Here we analyze by comparative genomics Pb mosquitocidal and non-mosquitocidal strains and show that the active component in Pbm responsible for Anopheles toxicity is a complex that contains a clostridial neurotoxin (CNT) that has high selectivity to anopheline mosquitoes, acquired through a megaplasmid. We found a second toxin locus (ptox) flanked by insertion sequences and transposon elements. This locus encodes a protein, which we named paraclostridial mosquitocidal protein 1 (PMP1), with high similarity to CNTs, a group that includes the tetanus neurotoxin (TeNT) and botulinum neurotoxins (BoNTs). PMP1’s closest relative is BoNT/X from C. botulinum strain 111 (36% identity), followed by BoNT/En, the Enterococcus BoNT-like protein7,9 (34% identity). PMP1 presents the conserved SxWY motif in the binding domain (HC), which in BoNTs is involved in ganglioside receptor binding (Supplemenatry Fig. 1C), as well as the conserved disulfide bond that links the toxin heavy and light chains, and is essential for toxicity. PMP1 is thus the first CNT that targets invertebrates.

To analyze if the SxWY motif is involved in toxicity and to determine the presence of other cell recognition regions, recombinant PMP1 HC was crystallized (residues 825–1260) and its structure determined at 1.95 Å resolution. PMP1 HC includes two subdomains, a N-terminal lectin-like fold (HCN) consisting primarily of 15 β-strands arranged in a jelly-roll fold and a C-terminal β-trefoil fold mostly composed of seven pairs of β-strands linked by loops (HCC). The HCC is the main region associated with cell recognition, and in PMP1, presents the most structural variation compared to other CNTs. One striking feature of PMP1 HCC is its general hydrophobicity, with an array of a dozen aromatic residues exposed on its surface and its lack of clear binding pockets. Of particular interest are the three extended loops found almost in parallel in the HCC subdomain. Extended loops 1094–1099 (loop 1), 1164–1172 (loop 2), and 1202–1208 (loop 3) present bulky hydrophobic side chains. A fourth loop composed of residues 1213–1222 (loop 4) was disordered, but seems to occupy a different position compared to the equivalent loops in BoNT/B and TeNT that are more protuberant. Remarkably, W1231A and W1224A mutations of the tandem SxWY motifs did not decrease toxicity. Instead, a similar motif, SWYG, located in loop 1 of the HC C terminus is critical, with an important role for the tryptophan in this loop. In addition, the mutant affecting a surface-exposed tyrosine hydrophobic patch (Y1100D/Y1101D/Y1173A/Y1227A) also nearly abolished toxicity.

> HHHHHHSQDPNALIDRLGIQLKDNLVFSLGVESDKIKDLSGNNTNLEVKTGVQIVDGRDSKTIRLNSNENSSIIVQKNESINFSYFSDFTISFWIRVPRLNKNDFIDLGIEYDLVNNMDNQGWKISLKDGNLVWRMKDRFGKIIDIITSLTFSNSFIDKYISSNIWRHITITVNQLKDCTLYINGDKIDSKSINELRGIDNNSPIIFKLEGNRNKNQFIRLDQFNIYQRALNESEVEMLFNSYFNSNILRDFWGEPLEYNKSYYMINQAILGGPLRSTYKSWYGEYYPYISRMRTFNVSSFILIPYLYHKGSDVEKVKIINKNNVDKYVRKNDVADVKFENYGNLILTLPMYSKIKERYMVLNEGRNGDLKLIQLQSNDKYYCQIRIFEMYRNGLLSIADDENWLYSSGWYLYSSGWYLDNYKTLDLKKHTKTNWYFVSEDEGWKE The system of five interrelated, functional β-lactamases stems from the recombination of two homologs, the TEM-1 penicillinase and the PSE-4 carbenicillinase. We further expand this investigation to engineered enzyme variants by examining the same range of motions in a closely interrelated system composed of three recombined and functionally selected variants of TEM-1 and PSE-4, or ‘chimeras’. We thus demonstrate that a variety of non-native slow motions, including active-site motions that occur near the frequency of turnover, are compatible with β-lactamase activity in engineered variants.

Among 32 natural variants of TEM-1 characterized to date for substitutions at position 68 and 69, Met68 can be mutated to Ile and Met69 to Ile/Leu/Val; the substitutions Met68Leu and the Met69Thr in the engineered cTEM-2m and cTEM-19m do not have natural counterparts. The inclusion of 17 substitutions left cTEM-17m essentially unaltered relative to TEM-1, but inclusion of the substitutions Met68Leu/Met69Thr in cTEM-2m and cTEM-19m dropped kcat 1 to 3 orders of magnitude, to levels similar to PSE-4. Finally, the Y105 active-site wall of cTEM-2m had an RMSF of 0.14 ± 0.05 nm (0.8–0.11 nm for the others), indicating ns-µs motions unique to this chimera. Among the 26 dynamic residues in cTEM-2m, we find 7 of the 11 dynamic residues of TEM-1. They are located in the active site and in the α/β domain, the latter containing the majority of the new dynamic residues of cTEM-2m. Thus, the slow motions of TEM-1 were generally maintained while additional residues acquired ms conformational exchange. Dynamic residues in cTEM-2m border and extend throughout the active-site wall 234–244 (Ile231, Lys234, Gly238 and residues 241–246), while TEM-1 showed a single dynamic residue there (Arg241).

>HPETLVKVKDAEDQLGARVGYIELDLNSGKILESFRPEERFPLTSTFKVLLCGAVLSRVDAGQEQLGRRIHYSQNDLVEYSPVTEKHLTDGMTVRELCSAAITMSDNTAANLLLTTIGGPKELTAFLHNMGDHVTRLDRWEPELNEAIPNDERDTTMPAAMATTLRKLLTGELLTLASRQQLIDWMEADKVAGPLLRSALPAGWFIADKSGAGERGSRGIIAALGPDGKPSRIVVIYTTGSQATMDERNRQIAEIGASLIKHW[2x]> DVYQEPTDPKFPQQWYLSGVTQRDLNVKAAWAQGYTGHGIVVSILDDGIEKNHPDLAGNYDPGASFDVNDQDPDPQPRYTQMNDNRHGTRCAGEVAAVANNGVCGVGVAYNARIGGVRMLDGEVTDAVEARSLGLNPNHIHIYSASWGPEDDGKTVDGPARLAEEAFFRGVSQGRGGLGSIFVWASGNGGREHDSCNCDGYTNSIYTLSISSATQFGNVPWYSEACSSTLATTYSSGNQNEKQIVTTDLRQKCTESHTGTSASAPLAAGIIALTLEANKNLTWRDMQHLVVQTSKPAHLNANDWATNGVGRKVSHSYGYGLLDAGAMVALAQNWTTVAPQRKCIIDILTEPKDIGKRLEVRKTVTACLGEPNHITRLEHAQARLTLSYNRRGDLAIHLVSPMGTRSTLLAARPHDYSADGFNDWAFMTTHSWDEDPSGEWVLEIENTSEANNYGTLTKFTLVLYGTASGSLVPRGSHHHH

Furin is one of the proprotein convertases (PCs), a family of subtilisin-like proteases involved in the maturation of many secreted proteins. PCs are Ca2+-dependent serine endoproteinases harboring a catalytic domain with structural homology to subtilisin. The so-called kexin/furin-like mammalian PC family members (furin, PC1, PC2, PC4, PACE4, PC5/6, and PC7) recognize multibasic substrate sequences and cleave after the common pattern (R/K)Xn(R)↓ (where n = 0, 2, 4, 6; X represents any amino acid; and “↓” marks the scissile peptide bond). The inhibitors induced a substantial conformational rearrangement of the active-site cleft by exposing a central buried tryptophan residue.

To investigate the binding mechanism of the (3,5-dichlorophenyl)pyridine-based inhibitors, we soaked compounds 1–5 into crystals of unliganded furin and solved the X-ray structures of the protease–inhibitor complexes. The displacement of Trp254 by the dichlorophenyl moiety and the interactions of the piperazine and piperidine as described for 1 were also observed for inhibitors 2–4, resulting in very similar binding poses. Accordingly, superpositions of the furin–inhibitor complexes with 1 and 2, 1 and 3, and 1 and 4 revealed very similar Cα root-mean-square deviation (RMSD) values of 0.04, 0.05, and 0.08 Å, respectively. Inhibitors 2, 3, and 4 contain negatively charged 2-methylbutanoic or propanoic acid substituents on the piperazine. Enzyme kinetics revealed similar or even higher potency of these inhibitors compared with 1. Interestingly, we found a well-defined water network that mediates interactions between the carboxylate groups of the inhibitors and positively charged residues of furin’s S1′ region. In contrast, for 3 and 4 one carboxylate oxygen interacts with two water molecules, adopting a favorable planar binding geometry. As the (3,5-dichlorophenyl)pyridine derivatives bind tightly to furin, we used single-cycle kinetic experiments to determine their off-rates. The dissociation of 1 and 3 from furin was slow (koff = (1.8 ± 0.6) × 10–4 s–1 and residence time τ = 92 min for 1; koff = (3.1 ± 2.2) × 10–4 s–1 and τ = 53.7 min for 3; Figure 2C and Table S3). The on-rates of 1 (kon = 4600 ± 2500 M–1 s–1) and 3 (kon = (9.6 ± 2.6) × 104 M–1 s–1) can be considered as slow and are likely to be influenced by a structural rearrangement needed for binding. A comparably high bioavailability of 2, 3, and 4 was reported in a bleomycin-induced lung fibrosis mouse model.> SNAMTPDFQIVTQRLQLRLITADEAEELVQCIRQSQTLHQWVDWCHALFSQQEAEQFIQATRLNWVKAEAYGFGVFERQTQTLVGMVAINEFYHTFNMASLGYWIGDRYQRQGYGKEALTALILFCFERLELTRLEIVCDPENVPSQALALRCGANREQLAPNRFLYAGE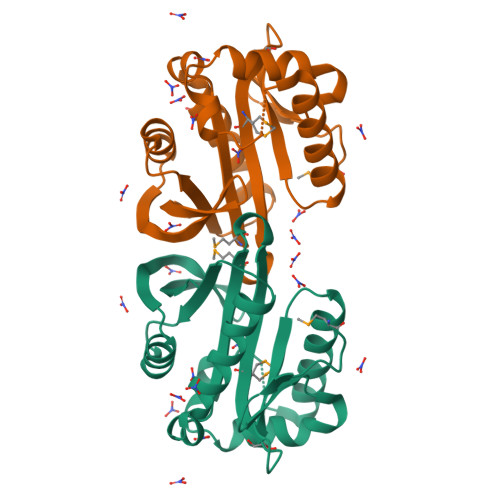PKAGIVFSLIP>[10x]IRVFAIPPSFASIFLTKSTKLTCLVTDLTTYDSVTISWTRQNGEAVKTHTNISESHPNATFSAVGEASICEDDWNSGERFTCTVTHTDLPSPLKQTISRPKGVALHRPDVYLLPPAREQLNLRESATITCLVTGFSPADVFVQWMQRGQPLSPEKYVTSAPMPEPQAPGRYFAHSILTVSEEEWNTGETYTCVVAHEALPNRVTERTVDKSTGKPTLYNVSLVMSDTAGTCY;> EDERIVLVDNKCKCARITSRIIRSSEDPNEDIVERNIRIIVPLNNRENISDPTSPLRTRFVYHLSDLCKKCDPTEVELDNQIVTATQSNICDEDSATETCYTYDRNKCYTAVVPLVYGGETKMVETALTPDACYPD;> KSPIFGPEEVNSVEGNSVSITCYYPPTSVNRHTRKYWCRQGARGGCITLISSEGYVSSKYAGRANLTNFPENGTFVVNIAQLSQDDSGRYKCGLGINSRGLSFDVSLEVSQGPGLLNDTKVYTVDLGRTVTINCPFKTENAQKRKSLYKQIGLYPVLVIDSSGYVNPNYTGRIRLDIQGTGQLLFSVVINQLRLSDAGQYLCQAGDDSNSNKKNADLQVLKPEPELVYEDLRGSVTFHCALGPEVANVAKFLCRQSSGENCDVVVNTLGKRAPAFEGRILLNPQDKDGSFSVVITGLRKEDAGRYLCGAHSDGQLQEGSPIQAWQLFVNEESTIPRSPTVVKGVAGGSVAVLCPYNRKESKSIKYWCLWEGAQNGRCPLLVDSEGWVKAQYEGRLSLLEEPGNGTFTVILNQLTSRDAGFYWCLTNGDTLWRTTVEIKIIEGEPNLKVPGNVTAVLGETLKVPCHFPCKFSSYEKYWCKWNNTGCQALPSQDEG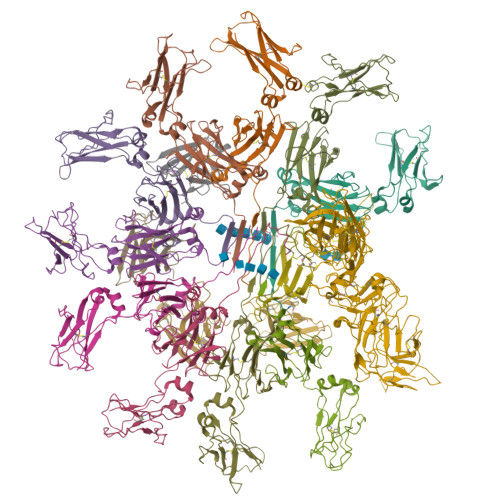PSKAFVNCDENSRLVSLTLNLVTRADEGWYWCGVKQGHFYGETAAVY;>RILPEVKVEGELGGSVTIKCPLPEMHVRIYLCREMAGSGTCGTVVSTTNFIKAEYKGRVTLKQYPRKNLFLVEVTQLTESDSGVYACGAGMNTDRGKTQKVTLNVHS[4x]> GDPVEDIIHDALGNTARRAISGATNVESAADTTPSSHRLETGRVPALQAAETGATSNATDENMIETRCVINRNGVLETTINHFFSRSGLVGVVNLTDGGDTTGYATWDIDIMGFVQLRRKCEMFTYMRFNAEFTFVTTTKSGEARPYMLQYMYVPPGAPKPTGRDAFQWQTATNPSVFVKLTDPPAQVSVPF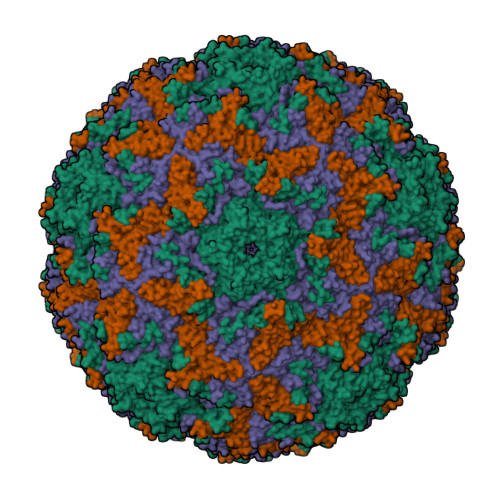MSPASAYQWFYDGYPTFGQHPETSNTTYGLCPNNMMGTFAVRVVSREASQLKLQTRVYMKLKHVRAWVPRPIRSQPYLLKNFPNYDSSKITNSARDRSSIKQANM;> SPSVEACGYSDRVAQLTVGNSSITTQEAANIVLAYGEWPEYCPDTDATAVDKPTRPDVSVNRFYTLDSKMWQENSTGWYWKFPDVLNKTGVFGQNAQFHYLYRSGFCLHVQCNASKFHQGALLVAVIPEFVIAGRGSNTKPNEAPHPGFTTTFPGTTGATFHDPYVLDSGVPLSQALIYPHQWVNLRTNNCATVIVPYINAVPFDSAINHSNFGLVVVPVSPLKYSSGATTAIPITITIAPLNSEFGGLRQAVSQ;> GIPAELRPGTNQFLTTDDDTAAPILPGFTPTPTIHIPGEVHSLLELCRVETILEVNNTTEATGLTRLLIPVSSQNKADELCAAFMVDPGRIGPWQSTLVGQICRYYTQWSGSLKVTFMFTGSFMATGKMLVAYSPPGSAQPANRETAMLGTHVIWDFGLQSSVSLVIPWISNTHFRTAKTGGNYDYYTAGVVTLWYQTNYVVPPETPGEAYIIAMGAAQDNFTLKICKDTDEVTQQAVLQ;> MGAQVSTQKSGSHETGNVATGGSTINFTNINYYKDSYAASATRQDFTQDPKKFTQPVLDSIRELSAPLN> GLKLDLTWFDKSTEDFKGEEYSKDFGDDGSVMESLGVPFKDNVNNGCFDVIAEWVPLLQPYFNHQIDISD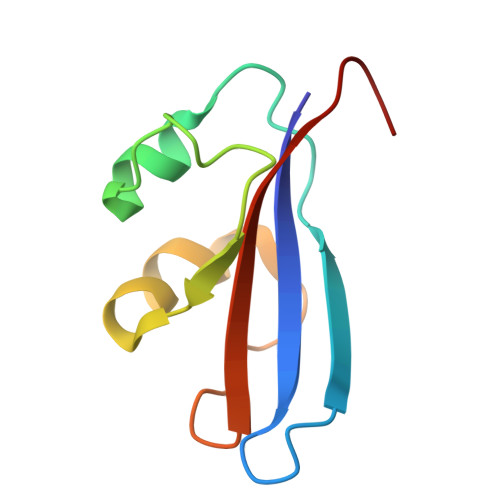NEYFVSFDYRDGDW>[4x]HHHHHHMQKQRTTSQWRE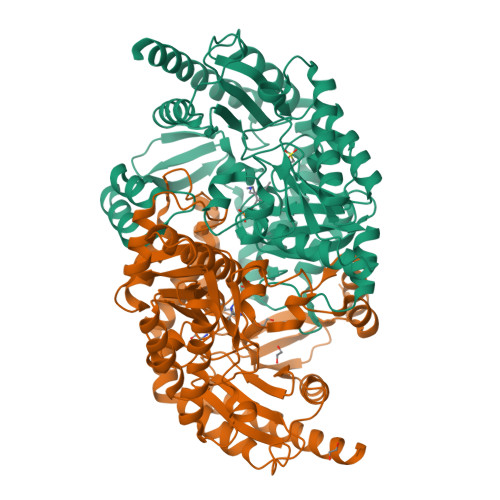LDAAHHLHPFTDTASLNQAGARVMTRGEGVYLWDSEGNKIIDGMAGLCCVNVGYGRKDFAEAARRQMEELPFYNTFFKTTHPAVVELSSLLAEVTPAGFDRVFYTNSGSESVDTMIRMVRRYWDVQGKPEKKTLIGRWNGYHGSTIGGASLGGMKYMHEQGDLPIPGMAHIEQPWWYKHGKDMTPDEFGVVAARWLEEKILEIGADKVAAFVGEPIQGAGGVIVPPATYWPEIERICRKYDVLLVADEVICGFGRTGEWFGHQHFGFQPDLFTAAKGLSSGYLPIGAVFVGKRVAEGLIAGGDFNHGFTYSGHPVCAAVAHANVAALRDEGIVQRVKDDIGPYMQKRWRETFSRFEHVDDVRGVGMVQAFTLVKNKAKRELFPDFGEIGTLCRDIFFRNNLIMRACGDHIVSAPPLVMTRAEVDEMLAVAERCLEEFEQTLKARGLA> GSGHWGAWMPSTISAFEGTCVSIPCRFDFPDELRPAVVHGVWYFNSPYPKNYPPVVFKSRTQVVHESFQGRSRLLGDLGLRNCTLLLSTLSPELGGKYYFRGDLGGYNQYTFSEHSVLDIVNTPNIVVPPEVVAGTEVEVSCMVPDNCPELRPELSWLGHEGLGEPTVLGRLREDEGTWVQVSLLHFVPTREANGHRLGCQAAFPNTTLQFEGYASLDVKYPPVIVEMNSSVEAIEGSHVSLLCGADSNPPPLLTWMRDGMVLREAVAKSLYLDLEEVTPGEDGVYACLAENAYGQDNRTVELSVMYAPWKPTVNGTVVAVEGETVSILCSTQSNPDPILTIFKEKQILATVIYESQLQLELPAVTPEDDGEYWCVAENQYGQRATAFNLSVEFAPIILLESHCAAARDTVQCLCVVKSNPEPSVAFELPSRN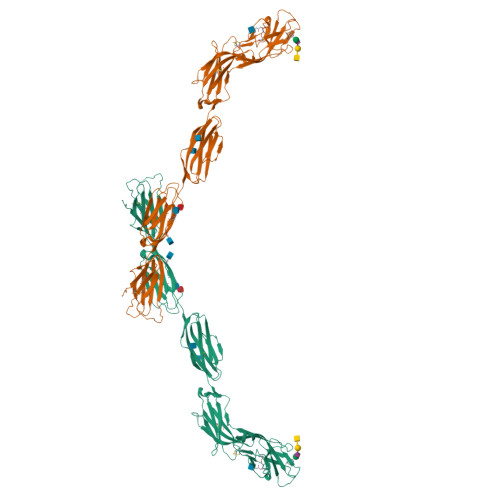VTVNETEREFVYSERSGLLLTSILTIRGQAQAPPRVICTSRNLYGTQSLELPFQGAHRAAAHHHHHH>SNASVERIYQKKTQLEHILLRPDTYIGSVELVTQQMWVYDEDVGINYREVTFVPGLYKIFDEILVNAADNKQRDPKMSCIRVTIDPENNLISIWNNGKGIPVVEHKVEKMYVPALIFGQLLTSSNYDDDEKKVTGGRNGYGAKLCNIFSTKFTVETASREYKKMFKQTWMDNMGRAGEMELKPFNGEDYTCITFQPDLSKFKMQSLDKDIVALMVRRAYDIAGSTKDVKVFLNGNKLPVKGFRSYVDMYLKDKLDETGNSLKVIHEQVNHRWEVCLTMSEKGFQQISFVNSIATSKGGRHVDYVADQIVTKLVDVVKKKNKGGVAVKAHQVKNHMWIFVNALIENPTFDSQTKENMTLQPKSFGSTCQLSEKFIKAAIGCGIVESILNWVKFKAQVQLN[2x]

Topoisomerase II (TOP2) enzymes are essential regulators of DNA topology during DNA transcription, replication, and repair. Topoisomerase IIβ (TOP2B) plays a role in transcriptional regulation and is expressed in all cell types including post-mitotic cardiomyocytes. Both isoforms catalyze the reaction, where one DNA duplex is passed through a transient double-strand DNA break in another DNA duplex. The ATPase domain of TOP2 is highly conserved between TOP2A and TOP2B and is composed of an N-terminal strap, a β-hairpin that is unique to eukaryotic TOP2, a GHKL ATPase domain that binds and hydrolyses ATP, and a transducer domain that conveys mechanical motion to the DNA binding and cleavage core of TOP2. Here we describe the development of the obex class of TOP2 inhibitors that bind to a previously unidentified druggable pocket in the TOP2 ATPase domain to act as allosteric catalytic inhibitors by locking the ATPase domain conformation with the capability of isoform-selective inhibition.

We co-crystallized the ATPase domains of TOP2A and TOP2B with 5c and the non-hydrolysable ATP analogue AMPPNP to identify the 5c binding site using X-ray crystallography. Compound 5c is clearly visible in a composite omit map in a binding site that is over 15 Å away from the nucleotide and dexrazoxane binding sites. 5c occupies the same binding pocket in both TOP2A and TOP2B, located at the nexus between the GHKL ATPase, transducer, and the 22 amino acid eukaryotic specific β-hairpin. Compound 5c consists of a substituted chromene core connected to a tetrahydroquinoline moiety via a non-planar amide linker. The chromene ring is buttressed between a Ser/Thr of the transducer domain and Met of the β-hairpin. The tetrahydroquinoline is accommodated within a hydrophobic pocket of the transducer domain. Most of the residues interacting with the core of 5c are similar between the two isoforms (R241, M61 and W62 for TOP2A; R257, M77 and W78 for TOP2B); however, subtle differences including a slight shift in conformation of 5c in TOP2A relative to TOP2B are likely associated with the non-conserved S320/T336 residues and a shift in the orientation of a GHKL Tyr residue (Y82/Y98) that extrudes from the top of this binding pocket. Interestingly, 5c induces a slight shift in Y72 of TOP2A compared to apo TOP2A due to packing of this non-conserved residue against the hydroxyethyl group, while the equivalent C88 residue in TOP2B is located 4.7 Å away and does not interact with 5c. The distance of 15 Å between the compound 5c and AMPPNP nucleotide binding sites suggests that 5c acts via an allosteric mechanism rather than as an ATP–competitive inhibitor. When bound to this site, 5c acts as an obstacle that would block the conformational change associated with ATP hydrolysis, which provides a mechanistic basis for TOP2 inhibition.> GPSGPCAKNSSIVGDSFKKAIRERQTVIYVQLRDACGDLLSSSIAATQPTSQALLPHQEPHSHLEQAMPTSDVQAFVISPDGSTVEVTMTPRENGIVALSYYPSIEGSYTLNILVKGTPISGCP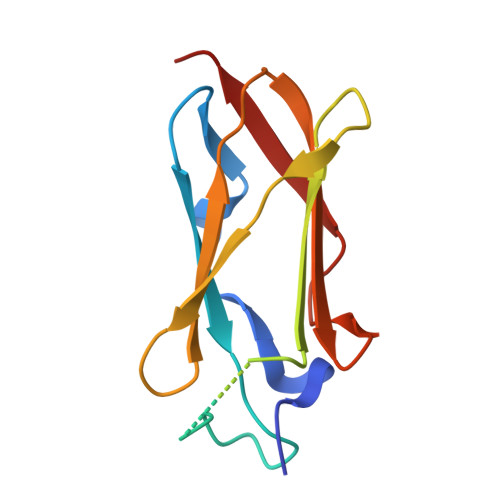TTMDIRRGR> MSEEVVQDAPLENNELNAEIDLQKTIQEEYKLWKQNVPFLYDLVITHALEWPSLTIQWLPDKKTIPGTDYSIQRLILGTHTSGNDQNYLQIASVQLPNFDEDTTEFTPSTIRRAQA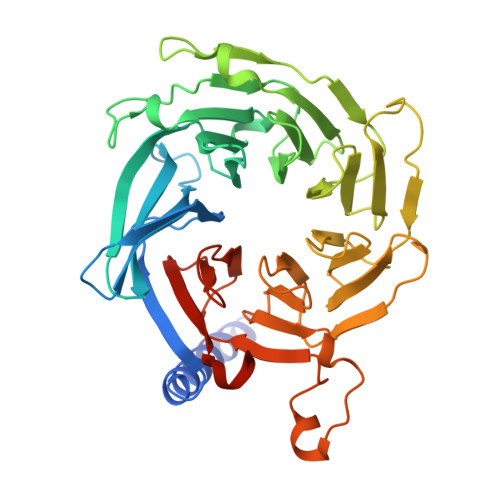TGSYTIEISQKIPHDGDVNRARYMPQKPEIIATMGEGGNAYIFDTTCHDALTTGEALPQAVLKGHTAEGFGLCWNPNLPGNLATGAEDQVICLWDVQTQSFTSSETKVISPIAKYHRHTDIVNDVQFHPQHEALLASVSDDCTLQIHDTRLNPEEEAPKVIQAHSKAINAVAINPFNDYLLATASADKTVALWDLRNPYQRLHTLEGHEDEVYGLEWSPHDEPILASSSTDRRVCIWDLEKIGEEQTPEDAEDGSPELLFMHGGHTNRISEFSWCPNERWVVGSLADDNILQIWSPSRVIWGRDHVQVSPRDLE> GAMADDEKNALPISKDGYIRVPKERVNVNLTSIKKLREKVDDSIHRELTDIFANLNYVGVVDEERRLAAIQHDLKLFLIDYGSVCYELFYQIGLTDFANFGKINLQSTNVSDDIVLYNLLSEFDELNDDASKEKIISKIWDMSSMLNEYYSIELVNDGLDNDLKS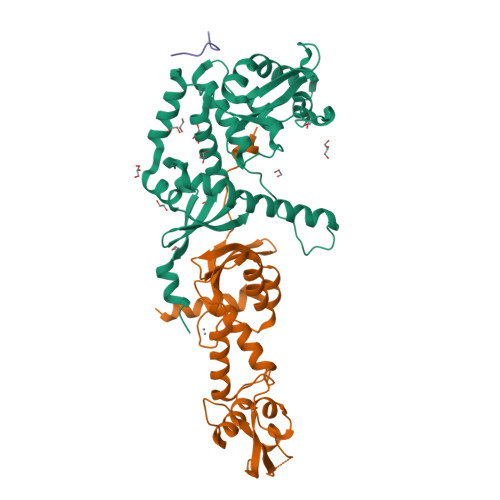VKLKSLPLLLKGYIPSLVKLPFFIYRLGKEVDWEDEQECLDGILREIALLYIPDMVPKVDTSDASLSEDEKAQFINRKEHISSLLEHVLFPCIKRRFLAPRHILKDVVEIANLPDLYKVFERC;> GSKRKSEAQENIIKNKDELEDFEQGEKYLTLTVSKNDFKKMEVVGQFNLGFIIVTRKVDNKYDLFIVDQHASDEKYNFETLQAVTVFKSQKLIIPQPVELSVIDELVVLDNLPVFEKNGFKLKIDEEEEFGSRVKLLSLPTSKQTLFDLGDFNELIHLIKEDGGLRRDNIRCSKIRSMFAMRACRSSIMIGKPLNKKTMTRVVHNLSELDKPWNCPHGRPTMRHLMELRDWSSFSKDYEI;> XVRSKYFKK We describe the design, kinetic properties, and structures of engineered subtilisin proteases that degrade the active form of RAS by cleaving a conserved sequence in switch 2. The engineering process to develop specificity for the RAS sequence QEEYSAM involved extensive modification of the Bacillus protease, subtilisin BPN’16–24, a canonical serine protease in which the scissile peptide bond is attacked by a nucleophilic serine (S221). The nucleophilicity of S221 results from its interactions with the catalytic histidine (H64) and aspartic acid (D32) that together form a charge relay system. To generate high specificity for the RAS target sequence, the active site was modified to be dependent on a cofactor (imidazole or nitrite) and protease sub-sites were engineered to create a linkage between substrate and cofactor binding.

To understand the structural basis for specificity and cofactor activation, we determined crystal structures of RASProtease(I) alone, in complex with YSAM and QEEYSAM product peptides, and with imidazole. An additional interesting feature of the structure of RASProtease(I) with QEEYSAM was the presence of an acyl adduct between the C-terminus of the P1 Met of the peptide and the Oγ of S221 of the enzyme. Apparently, the binding energy of the QEEYSAM peptide is sufficient to push its terminal carbon and Oγ of S221 into an orientation that drives the equilibrium from a product complex to the acyl enzyme. In particular, for the fully engineered RAS-specific proteases described here, binding of the cognate QEEYSAM sequence results in structural changes that are transmitted from the binding pockets to the active site and enable cofactor activation. Binding of the cognate substrate with a P4 tyrosine rescues the active conformation, however, by supplying stabilizing interactions in the S4 pocket that are transmitted to the catalytic region and promote productive binding of cofactor. Structures with a cognate peptide bound show that the L135V mutation allows space for an adventitious ion-binding site that coordinates the hydroxyl group of the P4 tyrosine of the substrate. This stabilizing interaction may be an important element for rescuing the active conformation of the catalytic region and enabling strong cofactor activation.

> EEYSAM;> AKCVSYGVAQIKAPALHSQGYTGSNVKVAILDTGIDSSHPDLNVAGGASFVPSETNPFQDNSSGGTHIAGTVLAVAPSASLYAVKVLGADGKGQASWIINGIEWAIANNMDVINMSLGSPSGSAAVKAAVDKAVASGVVVVAAAGNSGTSGSSSTVTYPAKYPSVIAVGAVDSSNQRAPFSSVGPELDVMAPGVSICSTLPGGKYGALSGTSMASPHVAGAAALILSKHPNWTNTQVRSSLENTATKLGDSFYYGKGLINVEAAAQ2-METHYLPROPAN-1-AMINE | 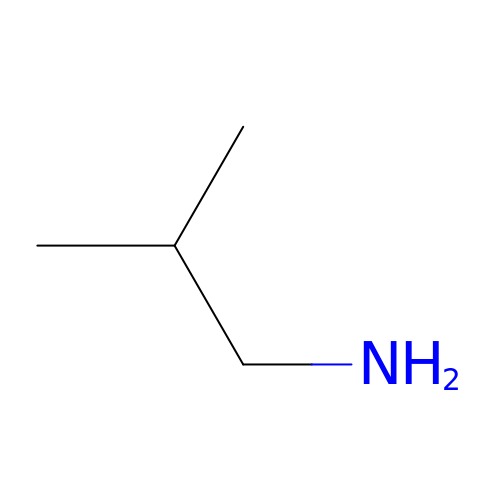C4 H11 N | KDSNLYIMUZNERS-UHFFFAOYSA-N> ENIEVHMLNKGAEGAMVFEPAYIKANPGDTVTFIPV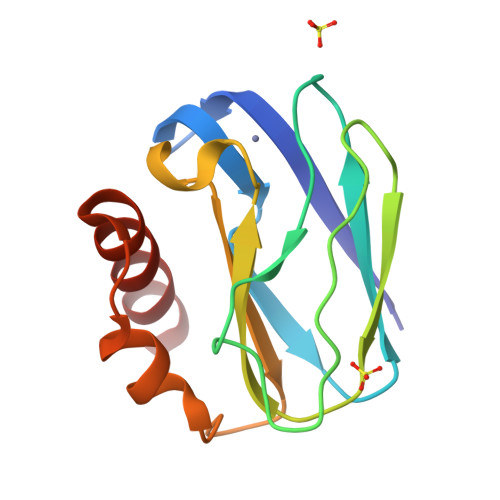DKGHNVESIKDMIPEGAEKFKSKINENYVLTVTQPGAYLVKCTPHYAMGMIALIAVGDSPANLDQIVSAKKPKIVQERLEKVIASAK> EWSHPQFEKGGKLTPKSINHPDIENYIAALQSDIANDLTMHYFKPLKNLPAIIPQYKTMTLNGDKVSNGIRNSYIESHIPAINGLSAGINIAMPNGESLFSIIIYVRRVINKASYRFLYETGPTIGINAKHEEVCTGKCPSPIPHQDGWVTFSKERSSNWGCEEWGCLAINDGCLYGSCQDIIRPEYKIYKKSSIEQKDVEVCITMAHESFCSTVDVLQPLISDRIQLDIQTIQMDSMPNIIAVKNGKVYVGDINDLGSTAKKCGSVQLYSEGIIGSGTPKFDYVCHAFNRKDVILRRCFDNSYQSCLLLEQDNTLTIASTSHMEVHKKVSSVGTINYKIMLGDFDYNAYSTQATVTIDEIRCGGCYGCPEGMACALKLSTNTIGSCSIKSNCDTYIKIIAVDPMQSEYSIKLNCPLATETVSVS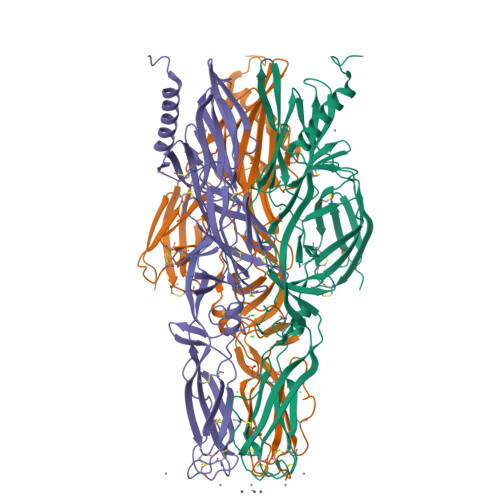VCSASAYTKPSI> GF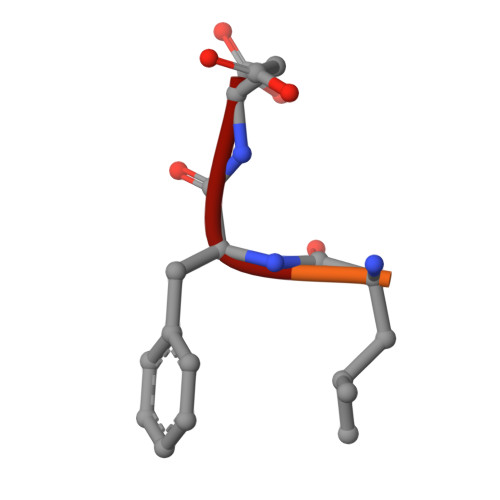GLFD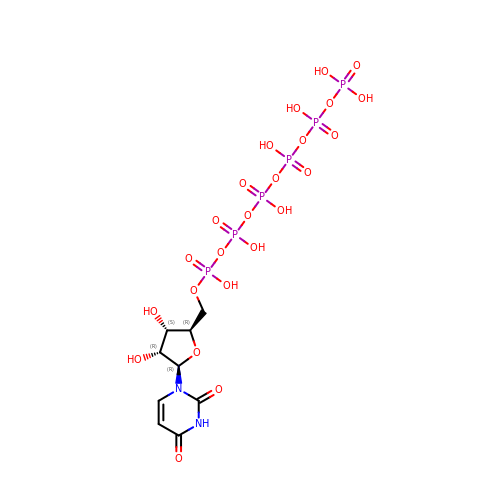5'-O-[(S)-hydroxy{[(S)-hydroxy{[(R)-hydroxy{[(S)-hydroxy{[(R)-hydroxy(phosphonooxy)phosphoryl]oxy}phosphoryl]oxy}phosphoryl]oxy}phosphoryl]oxy}phosphoryl]uridine | C9 H18 N2 O24 P6 | NJANLGXPTVMCFP-XVFCMESISA-N> XLTFAEY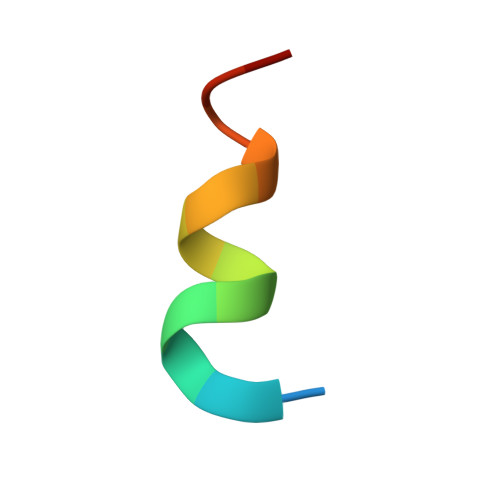WAQLASX D-CYSTEINE | 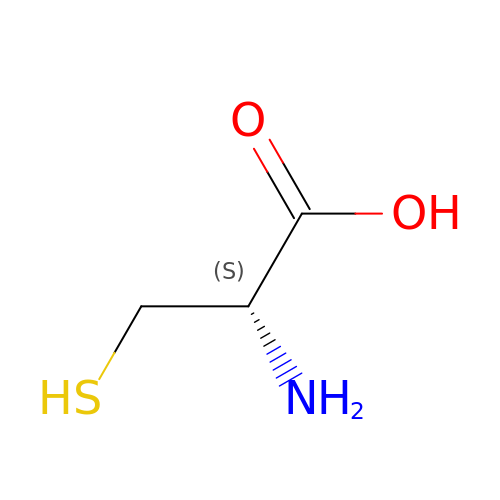C3 H7 N O2 S | XUJNEKJLAYXESH-UWTATZPHSA-N>MPNYKLTYFNMRGRAEIIRYIFAYLDIQYEDHRIEQADWPEIKSTLP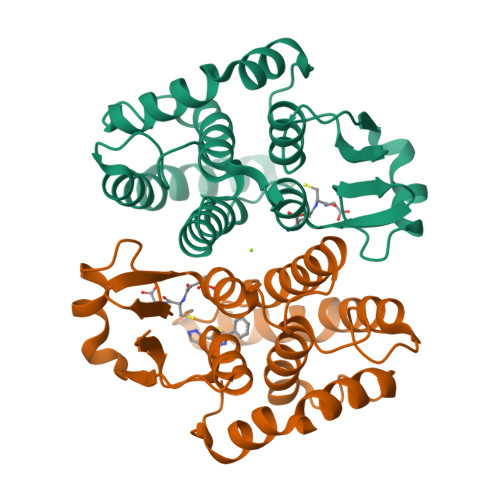FGKIPILEVDGLTLHQSLAIARYLTKNTDLAGNTEMEQCHVDAIVDTLDDFMSCFPWAEKKQDVKEQMFNELLTYNAPHLMQDLDTYLGGREWLIGNSVTWADFYWEICSTTLLVFKPDLLDNHPRLVTLRKKVQAIPAVANWIKRRPQTKL[4x]>[4x]SMTLYSDQELAYLQQGEEAMQKALGILSNQEGWKKESQQDNGDKVMSKVVPDVGKVFRLEVVVDQPMERLYEELVERMEAMGEWNPNVKEIKVLQKIGKDTFITHELAAEAAGNLVGPRDFVSVRCAKRRGSTCVLAGMATDFGNMPEQKGVIRAEHGPTCMVLHPLAGSPSKTKLTWLLSIDLKGWLPKSIINQVLSQTQVDFANHLRKRLESHPASEAR

Steroidogenic acute regulatory (StAR) protein related lipid transfer (START) domains are small globular modules that form a cavity where lipids and lipid hormones bind. The ∼210 residue globular START module is a curved β-sheet gripped by two α-helices. The concave face of the β-sheet and the C-terminal α-helix enclose a hydrophobic cavity that can accommodate lipid molecules. Here we present crystal structures of four human START domains, those of STARD1, STARD5, STARD13 and STARD14/ACOT11.

Group 1 contains the name-giving family member, steroidogenic acute regulatory protein (StAR/STARD1), and STARD3. Both are cholesterol carriers, and mutations in STARD1 cause congenital lipoid adrenal hyperplasia. In the StAR group there is a similar ion pair between the β–strands, namely, Glu169 and Arg188, which is not found in other family members that bind cholesterol. Arg188 has been suggested to bind to the hydroxyl group of cholesterol and it is also present in PCTP and RhoGAP groups. All structures reported are relevant to disease. They are down- (STARD13) or up-regulated (STARD5) in cancers, mutations in them result in metabolic disorders (STARD1) or they are linked to obesity (STARD14;).>SQDIVDFSQHPWKAPGPNDLRSPCPGLNTLANHGFLPRNGRNITIPMIVQAGFDGYNVQPDILILAAKVGLLTSPEPDTFTLDDLKLHGTIEHDASLSREDFALGDNLHFNEAIFNTLANSNPGSDVYNITSAGQVLKDRLADSLARNPNVTNTGKEFTIRTLESAFYLSVMGNATTGEAPKNFVQIFFREERLPIEEGWKRSTTPITSDTLNPIAGQISEASNWKPNPDQCPWIVLSPNL[2x]

Unspecific peroxygenases (UPOs) are a class of heme‐thiolate oxygenases from fungi that have similar catalytic scope to P450s, but are dependent only upon hydrogen peroxide (H2O2) as the external oxidant. A recent survey by Faiza and co‐workers explored the diversity of UPOs within sequence databases and was able to identify two major groups of enzymes: ‘long’ UPOs (Group I), typified by AaeUPO, of approximately 45 kDa molecular weight, and ‘short’ UPOs (Group II), typified by the enzyme from Marasmius rotula (MroUPO), which are of approximately 29 kDa. In this study, we have cloned the gene encoding an ‘artificial’ short UPO (artUPO) close in sequence to MroUPO, and expressed it in both Pichia pastoris and E. coli. In addition to their overall similarities in fold, artUPO, MroUPO and HspUPO feature both a glutamic acid and histidine residue (E164 and H93 in artUPO) that forms the catalytic acid‐base pair, in common with CPO and in contrast to the Glu‐Arg dyad found in AaeUPO.

We first crystallized artUPOyeast and determined the structure of the enzyme in two forms: the first in space group P212121, to a resolution of 2.01 Å and the second in C2221, to 1.21 Å, with two and one molecules in the asymmetric unit, respectively. Superimposition of the two, non‐equivalent, monomers in the P212121 structure give an rmsd of 0.21 Å over 231 C‐alpha atoms, suggesting that they are very similar. We cannot exclude the possibility of cooperativity in the mechanism of artUPO, although the kinetic plots presented are not suggestive of more than one phase in ligand binding. The structures confirm that each is a member of the short class of UPOs as defined by Faiza and co‐workers. Interestingly, despite the overall similarity of artUPO to HspUPO, the latter enzyme does not form a dimer, lacking the extended C‐terminal chain in artUPO that bears both C232 and W234 in artUPO. The side chain amine of K156 H‐bonds with the backbone carbonyl groups of G89 and T90 in artUPOyeast, and may also confer extra stability to the enzyme. The differences between the active site tunnels of artUPOyeast and AaeUPO‐PaDa‐I are also noteworthy. artUPOyeast is distinguished from AaeUPO by the replacement of characteristic phenylalanine residues in that enzyme with smaller or hydrophilic side chains including I91 for F121, L65 for F76 and K156 for F188, with G195 (common to AaeUPO and HspUPO) replaced by L163. Catalytic efficiency for the UPO substrate 5‐nitro‐1,3‐benzodioxole (NBD) was largely the same for both enzymes, and the structures also revealed few differences apart from the expected glycosylation of the yeast enzyme. However, the glycosylated enzyme displayed greater stability, as determined by nano differential scanning fluorimetry (nano‐DSF) measurements.> MTSADLTKPIEWPEMPVSLELQNAVEQFYYREAQLLDYQNYEAWLALLTQDIQYWMPIRTTHTSRNKAMEYVPPGGNAHFDET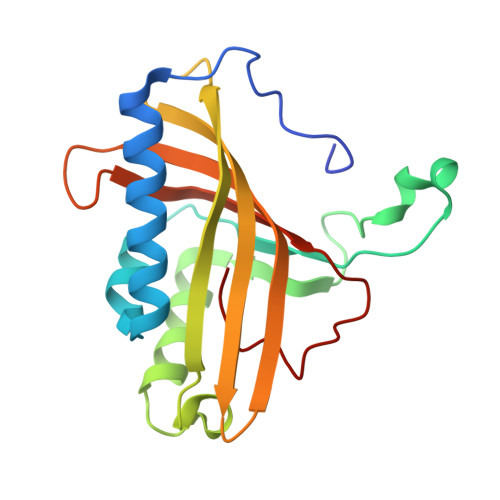YESMRARIRARVSGLNWTEDPPSRSRHIVSNVIVRETESAGTLEVSSAFLCYRNRLERMTDIYVGERRDILLRVSDGLGFKIAKRTILLDQSTITANNLSQFF>[2x]CC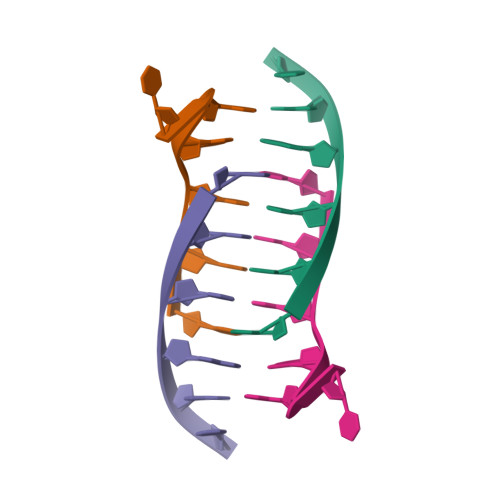CAAT>MRVITLAGSPRFPSRSSSLLEYAREKLNGLDVEVYHWNLQNFAPEDLLYARFDSPALKTFTEQLQQADGLIVATPVYKAAYSGALKTLLDLLPER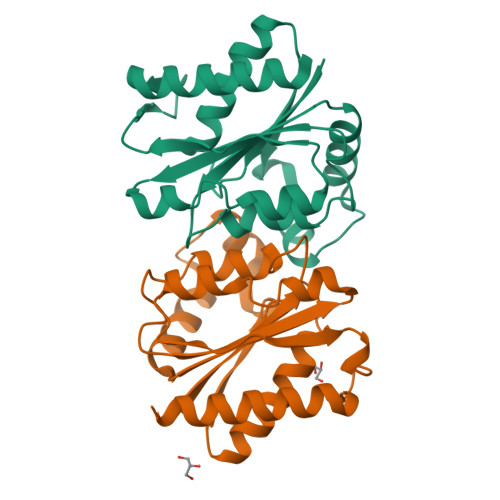ALQGKVVLPLATGGTVAHLLAVDALKPVLSALKAQEILHGVFADDSQVIDYHHRPQFTPNLQTRLDTALETFWQALHRRDVQVPDLLSLRGNAHA[2x]>GSEELLDLFNRQVTQEFTASQVYLSASIWFDQNDWEGMAAYMLAESAEEREHGLGFVDFANKRNIPIELQAVPAPVSCAEWSSPEDVWQSILELEQANTRSLLNLAEAASTCHDFAVMAFLNPFHLQQVNAEDKIGSILAKVTDENRTP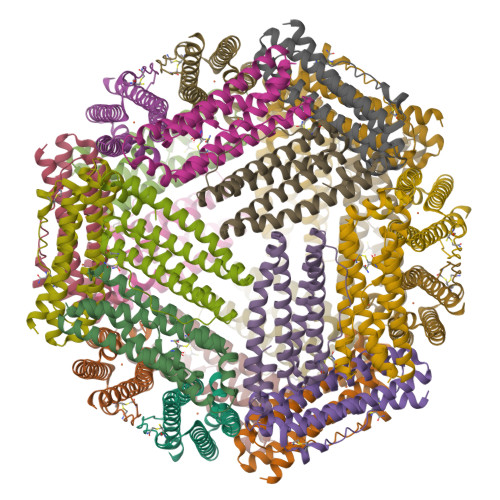GLLRSLDVVSFLGPCLFRS[8x]> DLICGTNYCKDHPCTSPIARAS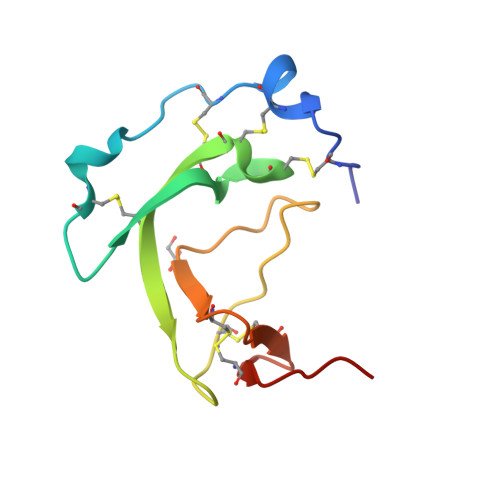CRSPATYRANHSGKCACCPACVTLLRERAACKTYSKEIGETPSAVCQEPLKCLNGVCTKVTPRR> SMASDMEEKFREAFILFSSCSDHIEM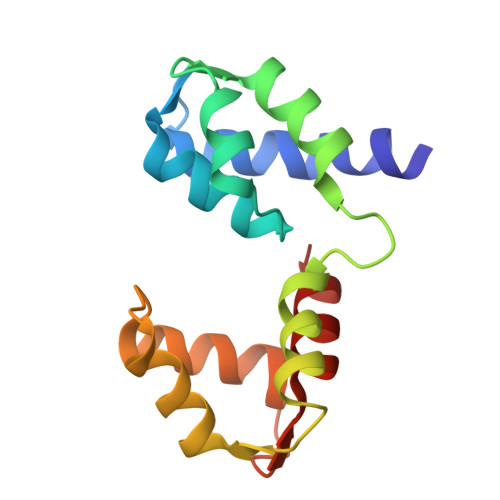YKFFELMNSFGIILTNDEKAALPNDINMDYWLNFAKKHYNYEQPFKHINNVNEQNTNVQIKIDNFLGIMKALDTRLTESDLNILLQITNPENKSTLNLKTVSQKLTESI> VRSLNSIVAVCQNMGIGKDGNLPWPPLRNEYKYFQRMTSTSHVEG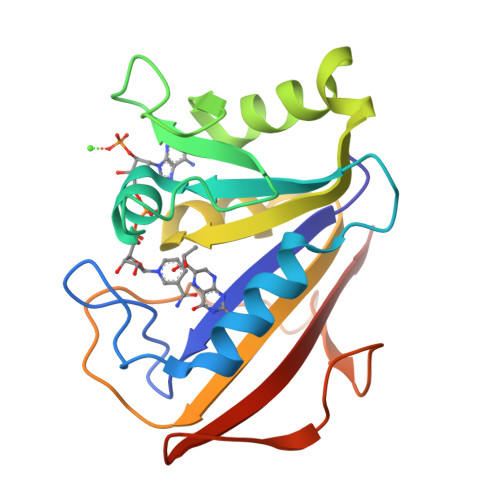KQNAVIMGKKTWFSIPEKNRPLKDRINIVLSRELKEAPKGAHYLSKSLDDALALLDSPELKSKVDMVWIVGGTAVYKAAMEKPINHRLFVTRILHEFESDTFFPEIDYKDFKLLTEYPGVPADIQEEDGIQYKFEVYQKSVLAQ> CTGCTGACTGTGGT;> GACCTGTA;> TACACCG;> CGGACAGTCA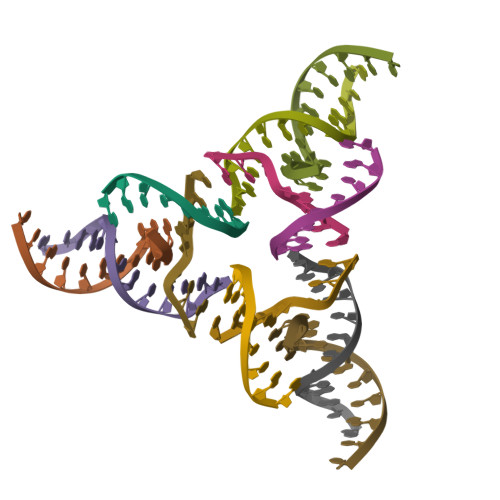GCA>[2x]MFQQLSARLQEAIGRLRGRGRITEEDLKATLREIRRALMDADVNLEVARDFVERVREEALGKQVLESLTPAEVILATVYEALKEALGGEARLPVLKDR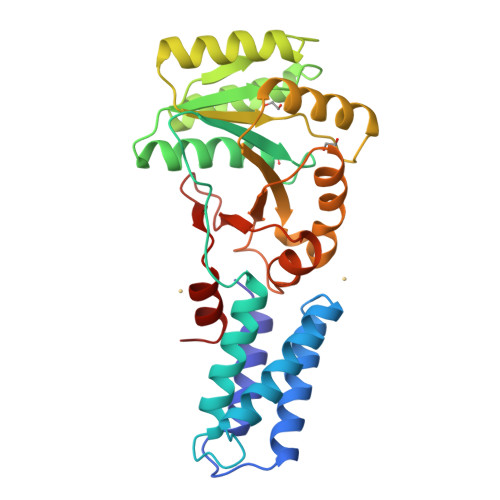NLWFLVGLQGSGKTTTAAKLALYYKGKGRRPLLVAADTQRPAAREQLRLLGEKVGVPVLEVMDGESPESIRRRVEEKARLEARDLILVDTAGRLQIDEPLMGELARLKEVLGPDEVLLVLDAMTGQEALSVARAFDEKVGVTGLVLTKLDGDARGGAALSARHVTGKPIYFAGVSEKPEGLEPFYPERLAGRILGM>GPGSMTETTTTFMDNVLGWLHKGYPEGVPPKDYFALLALLKRSLTEDEVVRAAQAILRSTDGQSPVTDDDIRNAVHQIIEKEPTAEEINQVA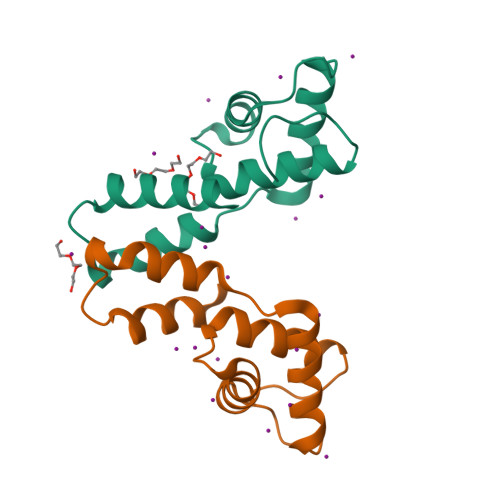ARLASVGWPLAVPVR[2x]3-HYDROXY-2-OXO-4-PHOPHONOXY- BUTYL)-PHOSPHONIC ACID 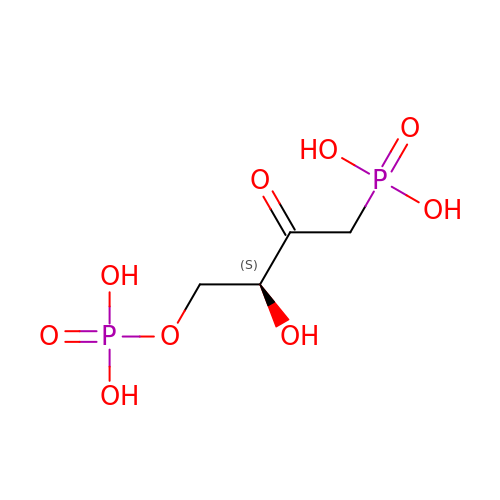| C4 H10 O9 P2 | ISHNYNQEXZYUQN-VKHMYHEASA-N>[7x]GPEESWEDDIAGQRTFPEDPNYPVMKSTFKSEYPFEKRKAESERIADRFPNRIPVICEKAEKSDIPEIDKRKYLVPADLTVGQFVYVIRKRIMLPPEKAIFIFVNDTLPPTAALMSAIYQEHKDKDGFLYVTYSGENTFG

Among them, the ubiquitin-like protein Atg8 (called LC3/GABARAP proteins in humans) plays a central role. In this study, we found that in both S. pombe and Saccharomyces cerevisiae, Atg8 physically interacts with Hfl1, a vacuole membrane protein. This interaction promotes the localization of Atg8 at the vacuole membrane in a lipidation-independent manner. hfl1Δ and atg8Δ caused the same vacuole-related phenotypes, which are not shared by other atg mutants. The structures showed that the Atg8-Hfl1 interaction is mediated by noncanonical mechanisms—using Hfl1 sequences adopting helical conformation (termed helical AIMs here) and in the case of budding yeast, involving a previously unreported binding site on Atg8.

Because a complex formed by ScAtg8 and ScHfl1(368-389) did not crystallize, we resorted to a fusion between them for crystallization, a strategy widely utilized for crystallization of a complex between an Atg8-family protein and a canonical AIM. The crystal structure of ScHfl1(368-389)-ScAtg8 fusion protein was determined at 2.45 Å resolution. The asymmetric unit of the crystal contains seven copies of the fusion protein, all of which form an intermolecular ScAtg8-ScHfl1(368-389) complex in a head-to-tail manner. Among the seven copies of ScHfl1(368-389), two have a slightly different conformation from the others due to crystal packing, while the other five copies have almost the same conformation; therefore, we use one representative structure of the ScAtg8-ScHfl1(368-389) complex from the five copies hereafter. ScHfl1(368-389) has an elongated conformation with a short helical conformation at the residues 374–377, and forms extensive interactions with the W-site, the L-site, α3, as well as β3 of ScAtg8, burying ~2400 Å2 of surface area (detailed interactions are summarized in Figure 3—figure supplement 3A). As is the case with SpHfl1, ScHfl1 neither forms an intermolecular β-sheet with Atg8 β2 (bottom), nor uses a canonical AIM sequence for binding to the W-site and the L-site. Instead, ScHfl1(368-389) uses Trp371 at the coil and Ile375 at the short helix for binding to the W-site and the L-site, respectively, with three residues between them. Unexpectedly, Tyr387 of ScHfl1 binds to a hydrophobic pocket formed between α3 and β3 of ScAtg8. This pocket, which has never been reported to be a binding site for AIMs, is named ‘Y-site’ because it accommodates a conserved Tyr residue in Hfl1. In addition to the hydrophobic interactions, electrostatic interactions are formed between the side-chains of Asp373, Asp374, and Asp384 of ScHfl1 and Arg28, Arg67, and Arg65 of ScAtg8, respectively, and as many as 12 hydrogen bonds are formed between ScHfl1 and ScAtg8 using both the main-chain and side-chain atoms.>MLKEVIPVNEITNFKSRAEEFFPIEWYKDMLHHHPVYYHEQTNTWNVFTYEGVKQVLGNYEFFSSAGPRTTIFVGANDKHEKASPLTNLTLVDPPDHRKGRSLLAAAFTPRSLKNWEPRIKQIAEELVENIQDNNEINIVEALAAPLPSMVIADLFGVPIQDRAQFKEWVDILFQPYDKERLEDIELQKQNAAKEYFQYLYPIVVQKRSNLSDDIISDLIQAEVDGEKFTDNEIVQVTMLLLGAGVETTSHAIANTFYSLLYDDESLYGELRNDLELVPNAVEEMLRYRFHMSRRDRTVKKDNNLLGVELKEGDVVIAWMSACNMDHRMFDDPFSINIHRPNNKKHLTFGNGPHFCLGAPLARLEMKIALETFVKKFSSIEPVEGFELEKNLTASATGQSLTNLPMNVYK[2x]

Cytochrome P450 (CYP) is a heme-containing enzyme that catalyzes hydroxylation reactions with various substrate molecules. Steroid hydroxylases are particularly useful for effectively introducing hydroxyl groups into a wide range of steroids in the pharmaceutical industry. This study reports a newly identified CYP steroid hydroxylase (BaCYP106A6) from the bacterium Bacillus sp. and characterizes it using an in vitro enzyme assay and structural investigation. The CYP106 and CYP109 families hydroxylate various types of steroids and terpenoids. Furthermore, NMR analysis of the chemical structures of the hydroxylated products of steroids indicated that the C15 region was the hydroxylation site by BaCYP106A6 with high regio- and stereoselectivity.

The crystal structure of BaCYP106A6 was determined at a 2.8-Å resolution using X-ray crystallography. The final model of BaCYP106A6 contained two monomers in the asymmetric unit, with the heme cofactor located at the center of each monomer. The two monomers form 2-fold rotational symmetry with a small interface area, which seems too small to form a realistic dimeric interface, indicating that BaCYP106A6 exists as a monomer. The monomeric structure of BaCYP106A6 consists of 17 α-helices and eight β strands and exhibits a typical fold seen in CYP monooxygenases with a centered heme cofactor molecule. The heme molecule is tightly bound to the central region of the BaCYP106A6 structure and is surrounded by α5, α12, α14, and α16 helices. The Cys356 residue is involved in the coordination of heme iron. The carboxyl groups of heme interact with the side chains of His97, Arg101, Arg297, and His354. The putative substrate-binding pocket is located directly above the heme molecule and consists of Ile72, His80, Asn88, Thr90, Leu240, Ala244, Thr248, Arg295, Ala396, and Thr397. In the case of Arg295, its side chain protrudes inside the binding pocket and occupies a large volume of the substrate-binding pocket in a substrate-free structure. Multiple sequence alignment indicated that the Arg295 residue is unique to the BaCYP106A6 sequence, and other CYP106 and CYP109 homologs do not have this positively charged residue at the corresponding position.>SNAKKKVLIYGAGSAGLQLANMLRQGKEFHPIAFIDDDRKKHKTTMQGITIYRPKYLERLIKKHCISTVLLAVPSASQVQKKVIIESLAKLHVEVLT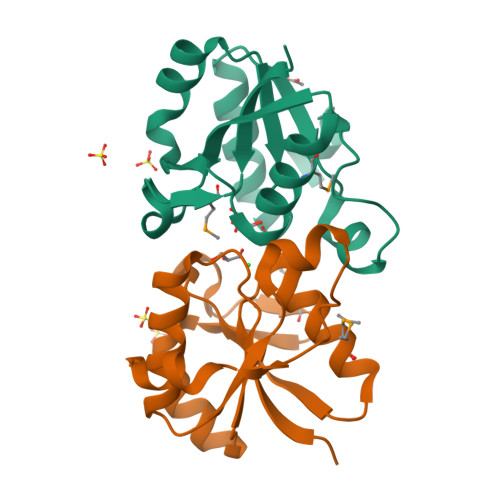IPNLDDLVNGKLSIGQLKEVSIDDLLGRVAVTPQAELMEANIKD[2x]(5-hydroxy-4-{[(7-hydroxy-6-oxo-2-phenyl-6,7-dihydro-2H-pyrazolo[3,4-b]pyridin-5-yl)amino]methyl}-6-methylpyridin-3-yl)methyl dihydrogen phosphate | 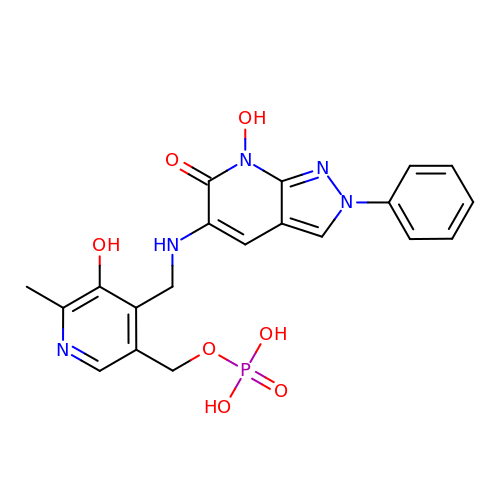C20 H20 N5 O7 P | FBCNGBFCTRTRCW-UHFFFAOYSA-N>[4x]MLKFMLDTNTCIFTIKNKPEHI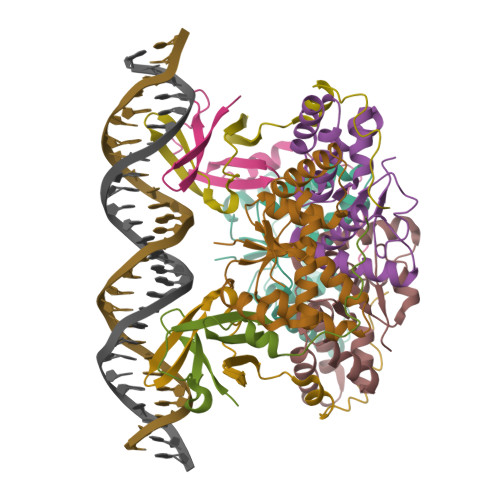RERFNLNTSRMCISSITLMELIYGAEKSLAPERNLAVVEGFISRLEVLDYDTQAAIHTGQIRAELARKGTPVGPYDQMIAGHAGSRGLVVVTNNLREFERIPGIRIEDWC;>MHTTLFFSNRTQAVRLPKSISFPEDVKHVEIIAVGRSRIITPVGESWDSWFDGEGASTDFMSTREQPA[4x]>MGSSHHHHHHSQDLASAEAGITGTWYNQSGSTFTVTAGADGNLTGQYENRAQGTGCQNSPYTLTGRYNGTKLEWRVEWNNSTENCHSRTEWRGQYQGGAEA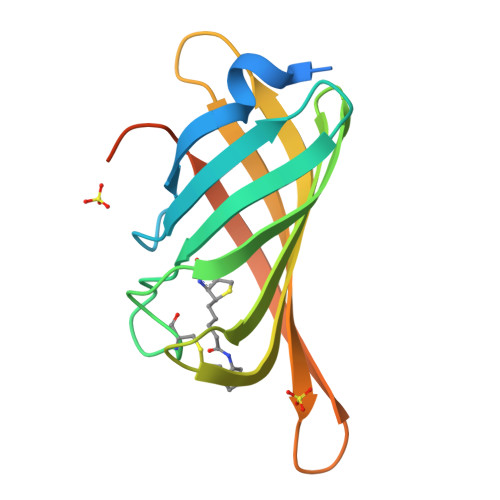RINTQWNLTYEGGSGPATEQGQDTFTKVKPSAASGSDYKDDDDK[6x]(10R)-10-methyl-3-(6-methylpyridin-3-yl)-9,10,11,12-tetrahydro-8H-[1,4]diazepino[5',6':4,5]thieno[3,2-f]quinolin-8-one | C21 H18 N4 O S | 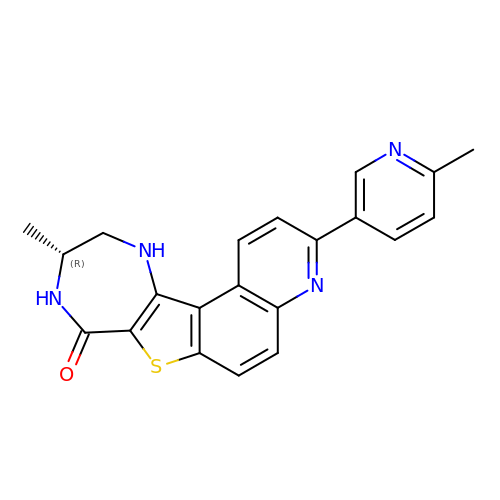CMWRPDHVGMHLSZ-GFCCVEGCSA-N>[2x]MPTKKQKSKSKLKPFFALVRRTNPSYGKLAFALALSVVTTLVSLLIPLLTKQLVDGFSMSNLSGTQIGLIALVFFVQAGLSAYATYALNYNGQKIISGLRELLWKKLIKLPVSYFDTNASGETVSRVTNDTMVVKELITTHISGFITGIISVIGSLTILFIMNWKLTLLVLVVVPLAALILVPIGRKMFSISRETQDETARFTGLLNQILPEIRLVKASNAEDVEYGRGKMGISSLFKLGVREAKVQSLVGPLISLVLMAALVAVIGYGGMQVSSGELTAGALVAFILYLFQIIMPMGQITTFFTQLQKSIGATERMIEILAEEEEDTVTGKQIENAHLPIQLDRVSFGYKPDQLILKEVSAVIEAGKVTAIVGPSGGGKTTLFKLLERFYSPTAGTIRLGDEPVDTYSLESWREHIGYVSQESPLMSGTIRENICYGLERDVTDAEIEKAAEMAYALNFIKELPNQFDTEVGERGIMLSGGQRQRIAIARALLRNPSILMLDEATSSLDSQSEKSVQQALEVLMEGRTTIVIAHRLSTVVDADQLLFVEKGEITGRGTHHELMASHGLYRDFAEQQLKMNADLENKAGVDKLAAALEHHHHHH

pmcATP-binding cassette (ABC) transporters are ubiquitous membrane proteins that couple the energy of ATP binding and hydrolysis to the translocation of a wide variety of molecules across biological membranes. Here, we investigated whether a large separation of the nucleotide-binding domains is required for the transport cycle of BmrA, a homodimeric multidrug ABC transporter from Bacillus subtilis. Upon ATP binding, the NBDs engage in a transient tight dimer where the two nucleotides are sandwiched between the Walker A motif from one NBD and the ABC signature motif from the other NBD, thereby generating the OF conformation that is prone to drug release. Overall, our data suggest that the NBDs of BmrA function with a tweezers-like mechanism distinct from the related lipid A exporter MsbA.

In order to rule out the possibility that the disulfide bond restrained a wider opening of BmrA, we also determined by cryo-EM the structure of the WT protein in the resting state at a resolution of 3.16 Å. The C-terminal domain of the transporter appears more flexible than the rest of the protein, and residues 578 onward could not be modeled. And on Movie S1, the structure of WT BmrA is highly similar to that of the A582C cross-linked mutant (rmsd of 0.86 Å over 931 residues). Both structures adopt an IF conformation where the whole NBDs are moderately separated. The transmembrane helices are perfectly superposed (rmsd of 0.45 Å over 549 residues) while the NBDs are slightly less separated in the mutant structure. However this difference is minimal and represents only 1.4 to 2.2 Å when comparing the Cα position of residues K351, K380, Q483, and H535 from the NBD conserved motifs (A-loop, Walker A motif, ABC signature, and H-loop, respectively) between the WT and the mutant proteins. In the absence of ligand, the distance between the spins was outside of measurable range (>60 Å), consistent with the BmrA IF cryo-EM structure where the Cα of the two cysteines are separated by 65 Å. By generating a molecular morph between the IF and OF conformations of WT BmrA, we found that the NBDs of the transporter can function according to a tweezers-like motion. In comparison, the NBDs of BmrA monomers are well aligned and dimerize in a single translation. Finally, we solved the first IF structure of BmrA, providing not only a structural framework for further experimental studies but also complementing the previously published OF structures of BmrA to further understand the molecular details of the alternating access transport mechanism.Phospholipases A2 (PLA2s) are the most abundant proteins found in Viperidae snake venoms and, in addition to their well-established ability to hydrolyze lysophospholipids in a calcium-dependent mechanism, these proteins can display toxic effects by different mechanisms. Despite their lack of enzymatic activity, Lys49-PLA2 myotoxins play a key role in myonecrosis, given that when they are selectively neutralized, most of the muscle-damaging effect of whole venoms is prevented. The muscle membrane-destabilizing activity exerted by Lys49-PLA2s has long been attributed to the presence of basic and aromatic residues situated at specific positions in the C-terminal region of these toxins (residues 115–129 according to the numbering system adopted by Renetseder and colleagues). In this work we report structural and functional studies concerning the mechanism through which RA neutralizes the in vitro inhibitory neuromuscular effect and muscle damage caused by PrTX-I, a Lys49-PLA2 from Bothops pirajai snake venom.

Crystals of the PrTX-I/RA complex diffracted X-rays to 1.77 Å resolution. The crystals belong to orthorhombic space group P212121, with unit-cell parameters a = 49.4 Å, b = 67.0 Å and c = 85.5 Å. Calculations based on the protein molecular weight indicate the presence of two molecules in the asymmetric unit. The homodimeric configuration adopted by Lys49-PLA2s has already been demonstrated by different techniques and is assumed to be the biological assembly in this study. The crystal structure of PrTX-I complexed to RA shows that the inhibitor interacts with the toxin at the entrance of its hydropohobic channel, demonstrating for the first time a ligand that interacts with this region of a Lys49-PLA2. Considering the mechanism proposed by dos Santos and colleagues, this finding suggests that the inhibitory effect of RA is the result of a steric hindrance that blocks the access of substrates to the hydrophobic channel. The fact that only one RA molecule was found to interact with the dimeric structure of PrTX-I can be rationalized by the presence of a PEG4000 molecule in the second hydrophobic channel, presumably arising from the high concentration of PEG4000 in the crystallization buffer combined with the high affinity of the channel for hydrophobic molecules. The blockade of one hydrophobic channel of the toxin (protomer A in this structure) by RA molecule occurs when the inhibitor interacts with atoms of both protomers, however conformational changes are observed only in the C-terminus of protomer B. The present data show that RA significantly reduces the blockade of indirectly evoked muscle contractions induced by PrTX-I by up to 90% and inhibits the muscle damage caused by this toxin in isolated phrenic-diaphragm preparations by about 80%.

>SLFELGKMILQETGKNPAKSYGAYGCNCGVLGRGKPKDATDRCCYVHKCCYKKLTGCNPKKDRYSYSWKDKTIVCGENNPCLKELCECDKAVAICLRENLGTYNKLYRYHLKPFCKKADDC[2x]Myriocin | C21 H39 N O6 | 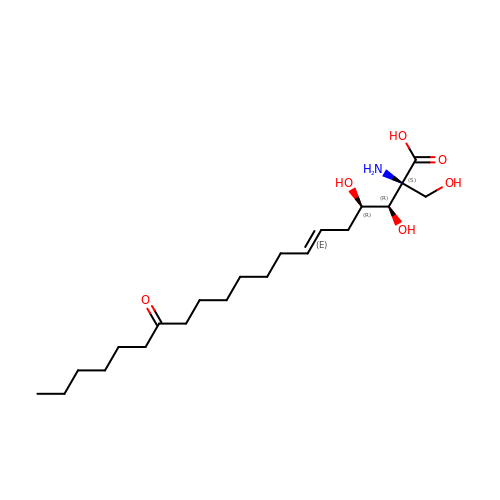ZZIKIHCNFWXKDY-GNTQXERDSA-N>[2x]GMEGLDKEKINKIIMEATKGSRFYGNELKKEKQVNQRIENMMQQKAQITSQQLRKAQLQVDRFAMELEQSRNLSNTIVHIDMDAFYAAVEMRDNPELKDKPIAVGSMSMLSTSNYHARRFGVRAAMPGFIAKRLCPQLIIVPPNFDKYRAVSKEVKEILADYDPNFMAMSLDEAYLNITKHLEERQNWPEDKRRYFIKMGSSVENDNPGKEVNKLSEHERSIS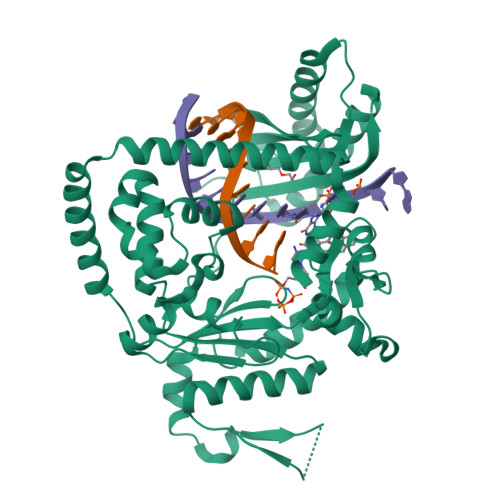PLLFEESPSDVQPPGDPFQVNFEEQNNPQILQNSVVFGTSAQEVVKEIRFRIEQKTTLTASAGIAPNTMLAKVCSDKNKPNGQYQILPNRQAVMDFIKDLPIRKVSGIGKVTEKMLKALGIITCTELYQQRALLSLLFSETSWHYFLHISLGLGSTHLTRDGERKSMSVERTFSEINKAEEQYSLCQELCSELAQDLQKERLKGRTVTIKLKNVNFEVKTRASTVSSVVSTAEEIFAIAKELLKTEIDADFPHPLRLRLMGVRISSFPN> GPTYKYLQKPMYEVQWKVVEEINGNNYVYIDPTQLPYDHKWEFPRNRLSFGKTLGAGAFGKVVEATAYGLIKSDAAMTVAVKMLKPSAHLTEREALMSELKVLSYLGNHMNIVNLLGACTIGGPTLVITEYCCYGDLLNFLRRKRDSFICSKTSPAIMEDDELALDLEDLLSFSYQVAKGMAFLASKNCIHRDLAARNILLTHGRITKICDFGLARDIKNDSNYVVKGNARLPVKWMAPESIFNCVYTFESDVWSYGI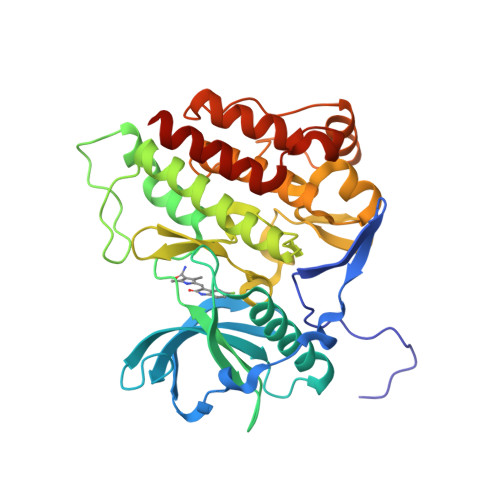FLWELFSLGSSPYPGMPVDSKFYKMIKEGFRMLSPEHAPAEMYDIMKTCWDADPLKRPTFKQIVQLIEKQISESTNHI>FDLEDVRPNQTAKAEKATTSYQDEETKKKTKEELDKLMEPTLGVEAKIPRRNRALFDKEGNRKATPDTTDELSEAQIMAIWNENIDEIPHLKELNDKTTSGLIYHSHDGKQEDKKRNLQYVRSGYVFDESYSEIVKNKNGVPYIFKNGIDGYIYYLGTSPSKELPKGNKVTYKGTWDFTSDVKTSYELSGFSDAGNGKNVAATSISDNVNRDHKVGEKLGDNEVKGVAHSSEFAVDFDNKKLTGSLYRNGYINRNKAQEVTKRYSIEADITGNRFRGKAKAEKAGDPIFTDSNYLEGGFYGPKAEEMAGKFFTNNKSLFAVFAAKSENGETTTERIIDATKIDLTQFNAKELNNFGDASVLIIDGQKIDLAGVNFKNSKTVEINGKTMVAVACCSNLEYMKFGQLWQKEGKQQVKDNSLFLQGERTATDKMPAGGNYKYVGTWDALVSKGTNWIAEADNNRESGYRTEFDVNFSDKKVNGKLFDKGGVNPVFTVDATINGNGFIGSAKTSDSGFALDAGSSQHGNAVFSDIKVNGGFYGPTAGELGGQFHHKSDNGSVGAVFGAKRQ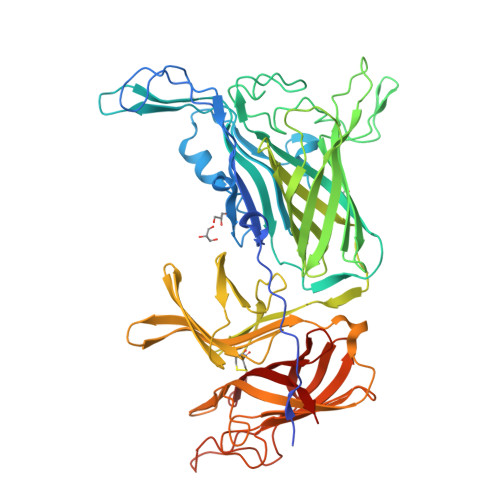IEK[2x]>[2x]GSHMANLDRTDDLVYLNVMELVRA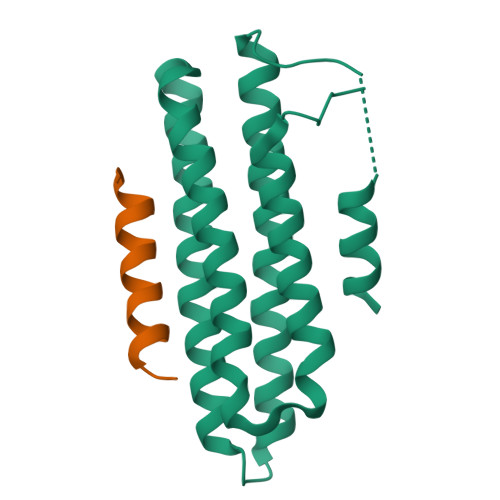VLELKNELSQLPPEGYVVVVKNVGLTLRKLIGSVDDLLPSLPSSSRTEIEGTQKLLNKDLAELINKMRLAQQNAVTSLSEEAKRQMLTASHTLAVDAKNLLDAVDQAKVLANLAHGGSGGGGGMEELDALLEELERSTLQDSD;>[2x]KTSAAAQLDELMAHLTEMQ> GMHSNINTLIANHRAGHALDQAFYTDAEVFQTDLQEIFYKEWLFAIPACELDKPGSYVTHQVGNYNVIIVRGADNVIRAFHNACRHRGSVICKAKKGNNPKLVCPYHQWTYELDGRLLWARDMGPDFEPSRHGLKTVHCRELAGLIYICLADEAPDFERFAEVARPYLEVHDLSNAKVAHESSIVERGNWKLVWENNRECYHCGGNHPALCRTFPDDPSVTGIEGGETPSNLQAHFDRCEQAGMPSGFHLSGDGQFRVARMPLKEGAESYTMDGKTAVRRWLGRAAFADAGS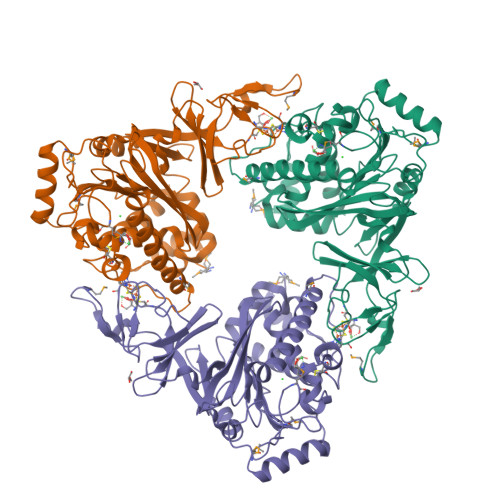LLKFHYPTTWNHFLSDHSIVFRVTPISPTETEVTTKWLVHKDAVEGVDYDLQRLTEVWIATNDEDREVVEFNQMGINSPAYEPGPYSPTQESGVLQFVEWYLSTLKRNSGPHAVAAE>[6x]MGHHHHHHHHHHSSGHIEGRHMADRLIVKGAREHNLRSVDLDLPRDALIVFTGLSGSGKSSLAFDTIFAEGQRRYVESLSAYARQFLGQMDKPDVDFIEGLSPAVSIDQKSTNRNPRSTVGTITEVYDYLRLLYARAGTPHCPTCGERVARQTPQQIVDQVLAMPEGTRFLVLAPVVRTRKGEFADLFDKLNAQGYSRVRVDGVVHPLTDPPKLKKQEKHDIEVVVDRLTVKAAAKRRLTDSVETALNLADGIVVLEFVDHELGAPHREQRFSEKLACPNGHALAVDDLEPRSFSFNSPYGACPECSGLGIRKEVDPELVVPDPDRTLAQGAVAPWSNGHTAEYFTRMMAGLGEALGFDVDTPWR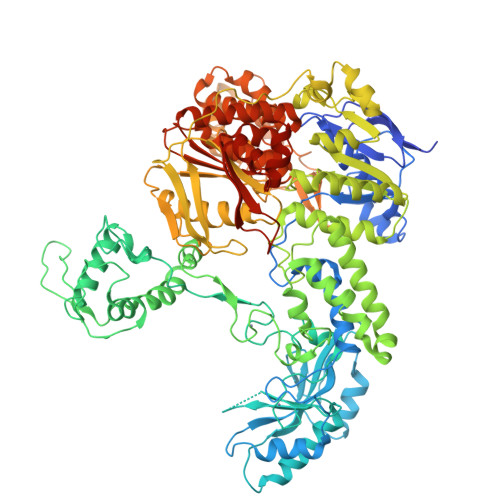KLPAKARKAILEGADEQVHVRYRNRYGRTRSYYADFEGVLAFLQRKMSQTESEQMKERYEGFMRDVPCPVCAGTRLKPEILAVTLAGESKGEHGAKSIAEVCELSIADCADFLNALTLGPREQAIAGQVLKEIRSRLGFLLDVGLEYLSLSRAAATLSGGEAQRIRLATQIGSGLVGVLYVLDEPSIGLHQRDNRRLIETLTRLRDLGNTLIVVEHDEDTIEHADWIVDIGPGAGEHGGRIVHSGPYDELLRNKDSITGAYLSGRESIEIPAIRRSVDPRRQLTVVGAREHNLRGIDVSFPLGVLTSVTGVSGSGKSTLVNDILAAVLANRLNGARQVPGRHTRVTGLDYLDKLVRVDQSPIGRTPRSNPATYTGVFDKIRTLFAATTEAKVRGYQPGRFSFNVKGGRCEACTGDGTIKIEMNFLPDVYVPCEVCQGARYNRETLEVHYKGKTVSEVLDMSIEEAAEFFEPIAGVHRYLRTLVDVGLGYVRLGQPAPTLSGGEAQRVKLASELQKRSTGRTVYILDEPTTGLHFDDIRKLLNVINGLVDKGNTVIVIEHNLDVIKTSDWIIDLGPEGGAGGGTVVAQGTPEDVAAVPASYTGKFLAEVVGGGASAATSRSNRRRNVSA>[2x]KDVTWEDIANDDKTTGDVLQYGMGTHAQRWSPLKQVNADNVFKLTPAWSYSFGDEKQRGQESQAIVSDGVIYVTASYSRLFALDAKTGKRLWTYNHRLPDDIRPCCDVVNRGAAIYGDKVFFGTLDASVVALNKNTGKVVWKKKFADHGAGYTMTGAPTIVKDGKTGKVLLIHGSSGDEFGVVGRLFARDPDTGEEIWMRPFVEGHMGRLNGKDSTVTGDVKAPSWPDDRNSPTGKVESWSHGGGAPWQSASFDAETNTIIVGAGNPGPWNTWARTAKGGNPHDYDSLYTSGQVGVDPSSGEVKWFYQHTPNDAWDFSGNNELVLFDYKAKDGKIVKATAHADRNGFFYVVDRSNGKLQNAFPFVDNITWASHIDLKTGRPVEREGQRPPLPEPGQKHGKAVE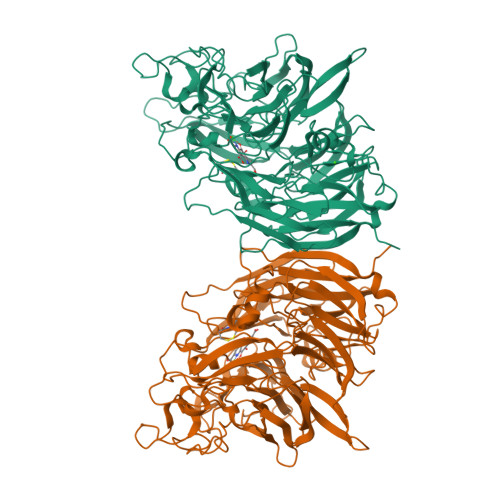VSPPFLGGKNWNPMAYSQDTGLFYVPANHWKEDYWTEEVSYTKGSAYLGMGFRIKRMYDDHVGSLRAMDPVSGKVVWEHKEHLPLWAGVLATAGNLVFTGTGDGYFKAFDAKSGKELWKFQTGSGIVSPPITWEQDGEQYLGVTVGYGGAVPLWGGDMADLTRPVAQGGSFWVFKLPSW>[2x]MNASLTPDQ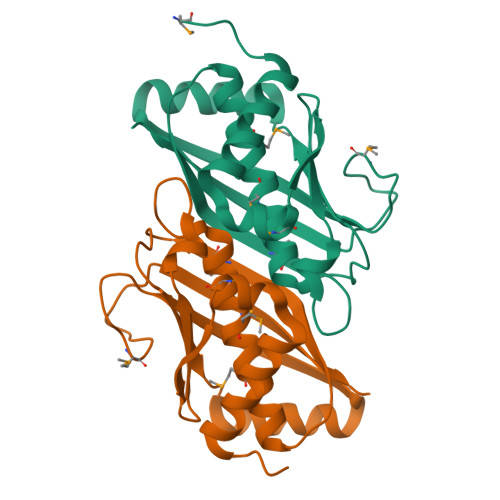VSKKLKQFFSDHLPISQFMGLEIESYDGDTLILTAPLEPNINDKQTAFGGSLYNAAVMACWGMVYLKTQEENIACNQVVTEGNMKYIAPVYGRIRAICHAPDEEELANFFDHFERKGKARISLEAAIYNDACVMKIEPETKPSVKFNGQYAILKNQ In addition, the cap fulfills numerous other biological functions that are mediated by specific cap-binding proteins and include maturation, transport, and eIF4E-mediated translation initiation. Upon binding the cap, the eIF4E protein changed its conformation from open to closed, bringing the Trp102 and Trp56 closer to the cap, and together with the structural water molecules, stapling the ligand with the protein structure. Finally, to gain more insight into the consequences at the molecular level of N7-benzylation of the mRNA cap, we determined the crystal structures of three compounds with eIF4E. Overall, the comparison of these three crystal structures indicated that different benzyl substituents can be accommodated in the cap binding pocket due to (i) the conformational flexibility of Trp102, which was also previously observed for m7GMP analogs, and (ii) the presence of structural water molecules in the N7-methyl-binding cavity, which could be replaced upon introduction of larger hydrophobic substituents.

One of the interesting examples is a dinucleotide cap analog carrying a benzyl group instead of methyl at the N7-position (Bn7GpppG). The modification slightly increased affinity for eIF4E, and when incorporated into mRNA, conferred almost twofold higher translation efficiency in vitro relative to m7GpppG-capped mRNAs, making it a good candidate for augmenting the properties of synthetic mRNAs. Crystal structures were refined using diffraction data to the resolution of 2.2 Å for 1a, 2.67 Å for 1c, and 2.66 Å for 1h. In the 1a–eIF4E complex the residue was flipped by 180° compared to the m7GpppG–eIF4E complex, but still participated in stacking interactions with modified guanine ring (the distance between the Bn7G plane and the parallelly aligned aromatic ring of Trp102 was approximately 3.5 Å). In the case of the benzyl modified cap 1a, for which the benzyl ring was directed upwards, most of the structural water molecules were conserved in the cavity, while for 3-MeBn7GpppG and 4-Cl-Bn7GpppG the benzyl rings were directed downwards into the cavity, and the structural water molecules were replaced by 3-methylbenzyl rings or 4-chlorobenzyl substituents. The guanosine of 4-Cl-Bn7GpppG was not visible in the crystal structure, while the guanosines of Bn7GpppG and 3-MeBn7GpppG were stabilized by interactions with amino acids from the loop comprised of residues 50–59. Specifically, backbone carbonyl oxygen atoms of lysine 54 and 52 formed hydrogen bonds with N1 and N2 of guanine, respectively, and amide group (NH2) of Asn59 was a donor in a hydrogen bond with O6 of guanosine.

>[2x]MVANPEHYIKHPLQNRWALWFFKNDKSKTWQANLRLISKFDTVEDFWALYNHIQLSSNLMPGCDYSLFKDGIEPMWEDEKNKRGGRWLITLNKQQRRSDLDRFWLETLLCLIGESFDDYSDDVCGAVVNVRAKGDKIAIWTTECENRDAVTHIGRVYKERLGLPPKIVIGYQSHADTATKSGSTTKNRFVV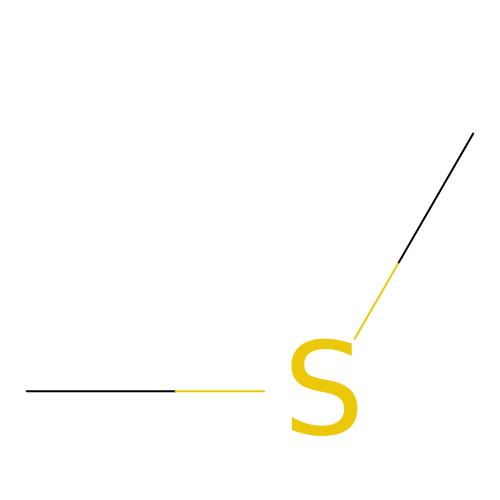(METHYLSULFANYL)METHANE | C2 H6 S | QMMFVYPAHWMCMS-UHFFFAOYSA-N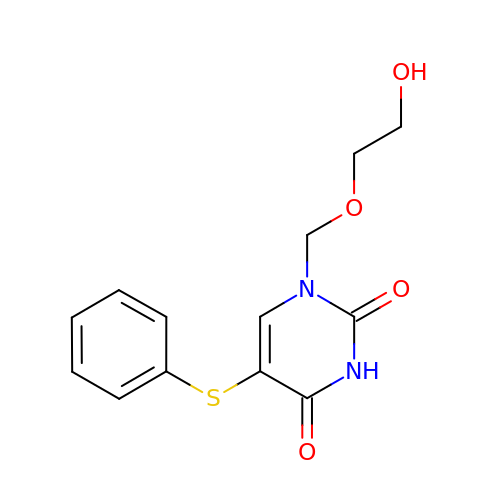1-((2-HYDROXYETHOXY)METHYL)-5-(PHENYLTHIO)PYRIMIDINE-2,4(1H,3H)-DIONE | C13 H14 N2 O4 S | YWJXYUXIPSIOGG-UHFFFAOYSA-N>[2x]GPLGSMASSNMKDETYYIALNM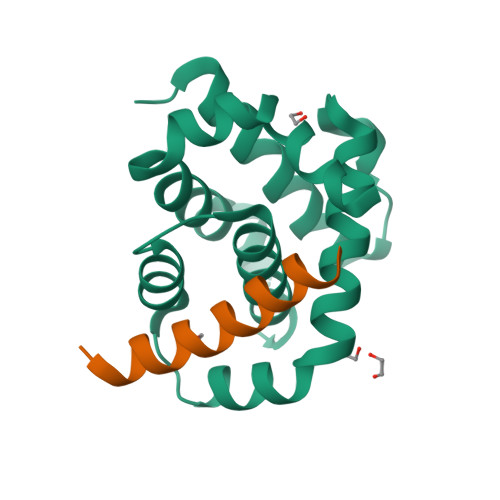IQNYIIEYNTNKPRKSFVIDSISYDVLKAACKSVIKTNYNEFDIIISRNIDFNVIVTQVLEDKINWGRIITIIAFCAYYSKKVKQDTSPQYYDGIISEAITDAILSKYRSWFIDQDYWNGIRIYKN;>[2x]EARTEVQIARKLQCIADQFHRLHIQR>[2x]MATATEQWVLVEMVQALYEAPAYHLILEGILILWIIRLLFSKTYKLQERSDLTVKEKEELIEEWQPEPLVPPVPKDHPALNYNIVSGPPSHKTVVNGKECINFASFNFLGLLDNPRVKAAALASLKKYGVGTCGPRGFYGTFDVHLDLEDRLAKFMKTEEAIIYSYGFATIASAIPA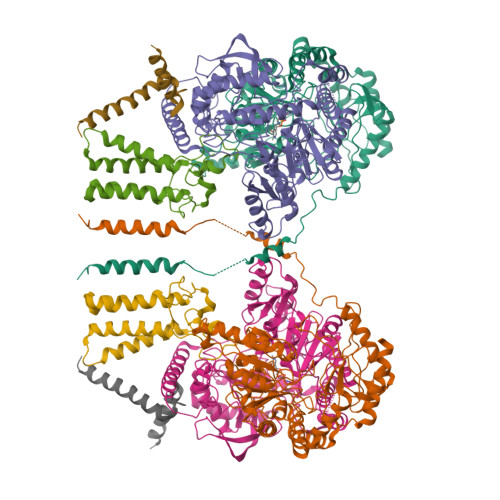YSKRGDIVFVDRAACFAIQKGLQASRSDIKLFKHNDMADLERLLKEQEIEDQKNPRKARVTRRFIVVEGLYMNTGTICPLPELVKLKYKYKARIFLEESLSFGVLGEHGRGVTEHYGINIDDIDLISANMENALASIGGFCCGRSFVIDHQRLSGQGYCFSASLPPLLAAAAIEALNIMEENPGIFAVLKEKCGQIHKALQGISGLKVVGESLSPAFHLQLEESTGSREQDVRLLQEIVDQCMNRSIALTQARYLEKEEKCLPPPSIRVVVTVEQTEEELERAASTIKEVAQAVLL;>[2x]MRPEPGGCCCRRTVRANGCVANGEVRNGYVRSSAAAAAAAAAGQIHHVTQNGGLYKRPFNEAFEETPMLVAVLTYVGYGVLTLFGYLRDFLRYWRIEKCHHATEREEQKDFVSLYQDFENFYTRNLYMRIRDNWNRPICSVPGARVDIMERQSHDYNWSFKYTGNIIKGVINMGSYNYLGFARNTGSCQEAAAKVLEEYGAGVCSTRQEIGNLDKHEELEELVARFLGVEAAMAYGMGFATNSMNIPALVGKGCLILSDELNHASLVLGARLSGATIRIFKHNNMQSLEKLLKDAIVYGQPRTRRPWKKILILVEGIYSMEGSIVRLPEVIALKKKYKAYLYLDEAHSIGALGPTGRGVVEYFGLDPEDVDVMMGTFTKSFGASGGYIGGKKELIDYLRTHSHSAVYATSLSPPVVEQIITSMKCIMGQDGTSLGKECVQQLAENTRYFRRRLKEMGFIIYGNEDSPVVPLMLYMPAKIGAFGREMLKRNIGVVVVGFPATPIIESRARFCLSAAHTKEILDTALKEIDEVGDLLQLKYSRHRLVPLLDRPFDETTYEETED;>MNVGTAHSEVNPNTRVMNSRGIWLSYVLAIGLLHIVLLSIPFVSVPVVWTLTNLIHNMGMYIFLHTVKGTPFETPDQGKARLLTHWEQMDYGVQFTASRKFLTITPIVLYFLTSFYTKYDQIHFVLNTVSLMSVLIPKLPQLHGVRIFGINKY[2x];>[2x]MADYKDDDDKSGPDEVDASGRMAGMALARAWKQMSWFYYQYLLVTALYMLEPWERTVFNSMLVSIVGMALYTGYVFMPQHIMAILHYFEIVQ>GSSGSSGMQLEIQVALNFIISYLYNKLPRRRVNIFGEELERLLKKKYEGHW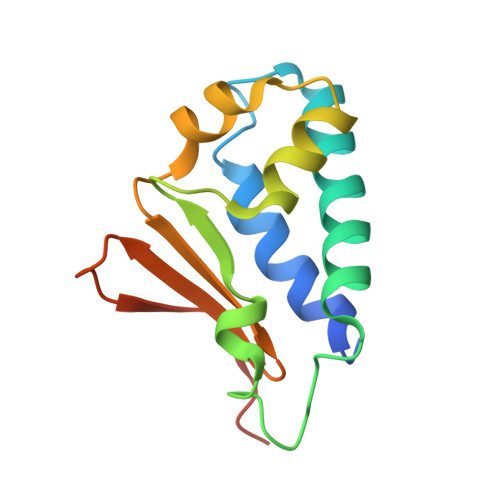YPEKPYKGSGFRCIHIGEKVDPVIEQASKESGLDIDDVRGNLPQDLSVWIDPFEVSYQIGEKGPVKVLYVDDNSGPSSG[4x]>MPVTEKDLAEDAPWKKIQQNTFTRWCNEHLKSVNKRIGNLQTDLSDGLRLIALLEVLSQKRMYRKYHQR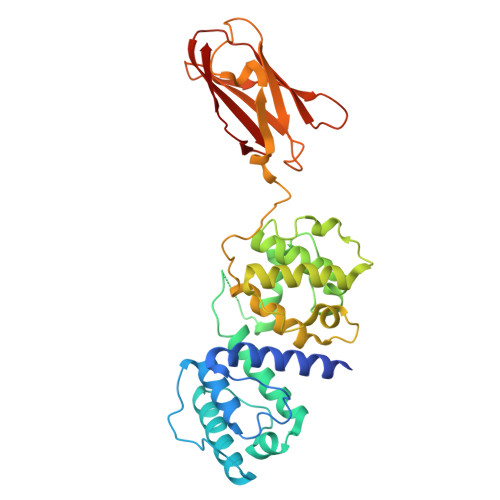PTFRQMQLENVSVALEFLDRESIKLVSIDSKAIVDGNLKLILGLVWTLILHYSISMPVWEDEGDDDAKKQTPKQRLLGWIQNKIPYLPITNFNQNWQDGKALGALVDSCAPGLCPDWESWDPQKPVDNAREAMQQADDWLGVPQVITPEEIIHPDVDEHSVMTYLSQFPKAKLKPGAPLKPKLNPKKARAYGRGIEPTGNMVKQPAKFTVDTISAGQGDVMVFVEDPEGNKEEAQVTPDSDKNKTYSVEYLPKVTGLHKVTVLFAGQHISKSPFEVSV[2x]N-SULFO-FLAVIN 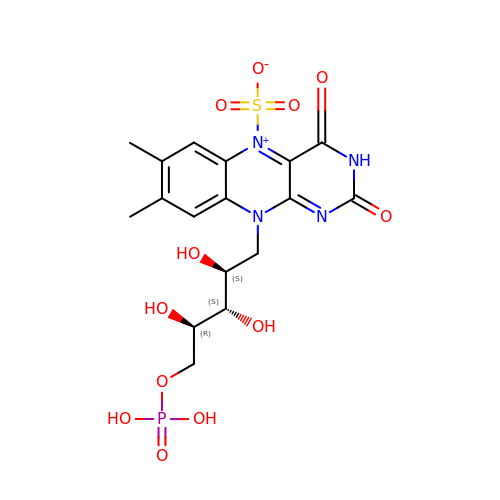MONONUCLEOTIDE | C17 H21 N4 O12 P S | ZLPUGFBBLGQWBS-SCRDCRAPSA-N> MGWSLPKEKGLILCLWNKFCRWFHRRESWAQSRDEQNLLQQKRIWESPLLLAAKENNVQALYKLLKFEGCEVHQKGAMGETALHIAALYDNNEAAQVLMEAAPELVFEPM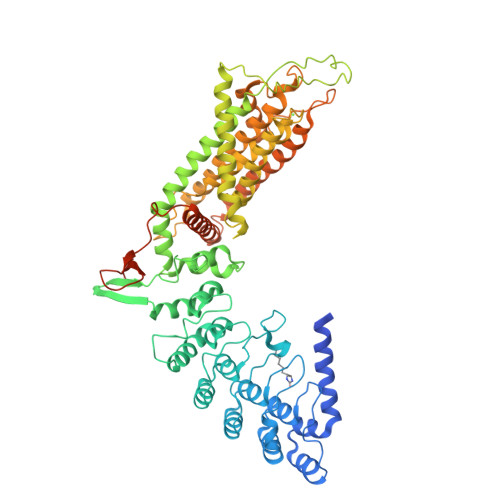TSELYEGQTALHIAVINQNVNLVRALLARGASVSARATGSVFHYRPHNLIYYGEHPLSFAACVGSEEIVRLLIEHGADIRAQDSLGNTVLHILILQPNKTFACQMYNLLLSYDGGDHLKSLELVPNNQGLTPFKLAGVEGNIVMFQHLMQKRKHIQWTYGPLTSTLYDLTEIDSSGDDQSLLELIVTTKKREARQILDQTPVKELVSLKWKRYGRPYFCVLGAIYVLYIICFTMCCVYRPLKPRITNRTNPRDNTLLQQKLLQEAYVTPKDDLRLVGELVSIVGAVIILLVEIPDIFRLGVTRFFGQTILGGPFHVIIVTYAFMVLVTMVMRLTNSDGEVVPMSFALVLGWCNVMYFARGFQMLGPFTIMIQKMIFGDLMRFCWQMAVVILGFASAFYIIFQTEDPDELGHFYDYPMALFSTFELFLTIIDGPANYDVDLPFMYSITYAAFAIIATLLMLNLLIAMMGDTHWRVAHERDELWRAQVVATTVMLERKLPRCLWPRSGICGREYGLGDRWFLRVEDRQDLNRQRIRRYAQAFQQQDDLYSEDLEKDSGEK> NCSKIHLSTKLLAVDFPAHFVKSISCQICEHILADPVETSCKHLFCRICILRCLKVMGSYCPSCRYPCFPTDLESPVKSFLNILNSLMVKCPAQDCNEEVSLEKYNHHVSSHKESKETLVHINKGGRPRQHLLSLTRRAQKHRLRELKIQVKEFADKEEGGDVKAVCLTLFLLALRARNEHRQADELEAIMQGRGSGLQPAVCLAIRVNTFLSCSQYHKMYRTVKAITGRQIFQPLHALRNAEKVLLPGYHPFEWQPPLKNVSSRTDVGIIDGLSGLASSVDEYPVDTIAKRFRYDSALVSALMDMEEDILEGMRSQDLDDYLNGPFTVVVKESCDGMGDVSEKHGSGPAVPEKAVRFSFTVMRITIEHGSQNVKVFEEPKPNSELCCKPLCLMLADESDHETLTAILSPLIAEREAMKSSELTLEMGGIPRTFKFIFRGTGYDEKLVREVEGLEASGSVYICTLCDTTRLEASQNLVFHSITRSHAENLQRYEVWRSNPYHESVEELRDRVKGVSAKPFIETVPSIDALHCDIGNAAEFYKIFQLEIGEVYKHPNASKEERKRWQATLDKHLRKRMNLKPIMRMNGNFARKLMTQETVD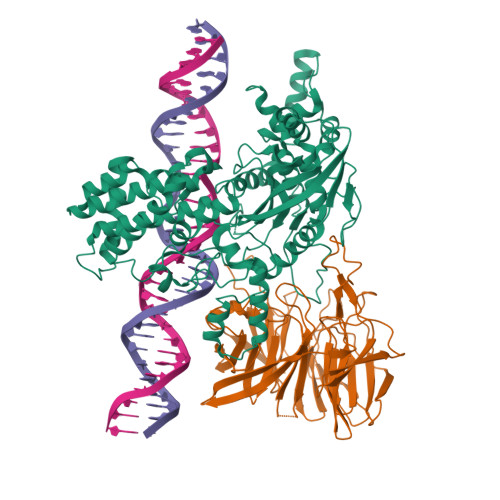AVCELIPSEERHEALRELMDLYLKMKPVWRSSCPAKECPESLCQYSFNSQRFAELLSTKFKYRYEGKITNYFHKTLAHVPEIIERDGSIGAWASEGNESGNKLFRRFRKMNARQSKCYEMEDVLKHHWLYTSKYLQKFMNAHNALKSSGFTMNSKETLGDPLGIEDSLESQDSME;> MSLQMVTVGHNIALIQPGFSLMNFDGQVFFFGQKGWPKRSCPTGVFHFDIKQNHLKLKPAIFSKDSCYLPPLRYPATCSYKGSIDSDKHQYIIHGGKTPNNELSDKIYIMSVACKNNKKVTFRCTEKDLVGDVPEPRYGHSIDVVYSRGKSMGVLFGGRSYMPSTQRTTEKWNSVADCLPHVFLIDFEFGCATSYILPELQDGLSFHVSIARNDTVYILGGHSLASNIRPANLYRIRVDLPLGTPAVNCTVLPGGISVSSAILTQTNNDEFVIVGGYQLENQKRMVCSLVSLGDNTIEISEMETPDWTSDIKHSKIWFGSNMGNGTIFLGIPGDNKQAMSEAFYFYTLRCSEEDLSEDQKIVSNSQTSTEDPGDSTPFEDSEEFCFSAEATSFDGDDEFDTYNEDDEDDESVTGYWITCCPTCDVDINTWVPFYSTELNKPAMIYCSHGDGHWVHAQCMDLEERTLIHLSEGSNKYYCNEHVQIARALQAPKRNPPLQKPPMKSLHKKGSGKVLTPAKKS>MSDREFVTVDPVTIIIKECINLSTAMRKYSKFTSQSGVAALLGGGSEIFSNQDDYLAHTFNNLNTNKHNDPFLSGFIQLRLMLNKLKNLDNIDSLTILQPFLLIVSTSSISGYITSLALDSLQKFFTLNIINESSQNYIGAHRATVNALTHCRFEGSQQLSDDSVLLKVVFLLRSIVDSPYGDLLSNSIIYDVLQTILSLACNNRRSEVLRNAAQSTMIAVTVKIFSKLKTIEPVNVNQIYINDESYTNDVLKADTIGTNVESKEEGSQEDPIGMKVNNEEAISEDDGIEEEHIHSEKSTNGAEQLDIVQKTTRSNSRIQAYADDNYGLPVVRQYLNLLLSLIAPENELKHSYSTRIFGLELIQTALEISGDRLQLYPRLFTLISDPIFKSILFIIQNTTKLSLLQATLQLFTTLVVILGNNLQLQIELTLTRIFSILLDDGTANNSSSENKNKPSIIKELLIEQISILWTRSPSFFTSTFINFDCNLDRADVSINFLKALTKLALPESALTTTESVPPICLEGLVSLVDDMFDHMKDIDREEFGRQKNEMEILKKRDRKTEFIECTNAFNEKPKKGIPMLIEKGFIASDSDKDIAEFLFNNNNRMNKKTIGLLLCHPDKVSLLNEYIRLFDFSGLRVDEAIRILLTKFRLPGESQQIERIIEAFSSAYCENQDYDPSKISDNAEDDISTVQPDADSVFILSYSIIMLNTDLHNPQVKEHMSFEDYSGNLKGCCNHKDFPFWYLDRIYCSIRDKEIVMPEEHHGNEKWFEDAWNNLISSTTVITEIKKDTQSVMDKLTPLELLNFDRAIFKQVGPSIVSTLFNIYVVASDDHISTRMITSLDKCSYISAFFDFKDLFNDILNSIAKGTTLINSSHDDELSTLAFEYGPMPLVQIKFEDTNTEIPVSTDAVRFGRSFKGQLNTVVFFRIIRRNKDPKIFSKELWLNIVNIILTLYEDLILSPDIFPDLQKRLKLSNLPKPSPEISINKSKESKGLLSTFASYLKGDEEPTEEEIKSSKKAMECIKSSNIAASVFGNESNITADLIKTLLDSAKTEKNADNSRYFEAELLFIIELTIALFLFCKEEKELGKFILQKVFQLSHTKGLTKRTVRRMLTYKILLISLCADQTEYLSKLINDELLKKGDIFTQKFFATNQGKEFLKRLFSLTESEFYRGFLLGNENFWKFLRKVTAMKEQSESIFEYLNESIKTDSNILTNENFMWVLGLLDEISSMGAVGNHWEIEYKKLTESGHKIDKENPYKKSIELSLKSIQLTSHLLEDNNDLRKNEIFAIIQALAHQCINPCKQISEFAVVTLEQTLINKIEIPTNEMESVEELIEGGLLPLLNSSETQEDQKILISSILTIISNVYLHYLKLGKTSNETFLKILSIFNKFVEDSDIEKKLQQLILDKKSIEKGNGSSSHGSAHEQTPESNDVEIEATAPIDDNTDDDNKPKLSDVEKD[2x]

The budding yeast homologs of GBF1, named Gea1 and Gea2, localize to early and medial Golgi compartments where Arf1 activation orchestrates the formation of COPI vesicles destined for the ER and earlier Golgi compartments. Here we present cryoelectron microscopy (cryoEM) structures of full-length Gea2, the yeast paralog of the human Arf-GEF GBF1, that reveal the organization of these regulatory domains and explain how Gea2 binds to the Golgi membrane surface. Gea2 and its paralogs possess an N-terminal DCB-HUS regulatory domain and C-terminal HDS1, HDS2, and HDS3 regulatory domains. The HDS1, −2, and −3 domains form an extended helical repeat structure that is contiguous with the DCB-HUS domain, such that the HDS3 domains of each monomer lie at the distal ends of the homodimer.

Three-dimensional classification of the particles revealed three distinct conformations of Gea2 homodimers that differed only in the positioning of the GEF domain, with each monomer adopting either a “closed” or “open” position relative to the regulatory domains. Based on the relative numbers of particle images that sorted into each of these three classes (~30% “closed/closed,” ~30% “open/open,” and ~40% “closed/open”), the conformation adopted by each monomer within the dimer appears to be largely independent of that of its binding partner. We begin our description of the structure using the “closed/open” dimer, as it exhibits both the closed and open states of the GEF domain. Unexpectedly, the GEF domain of Gea2 adopts two conformational states. The GEF domain lies adjacent to the HUS domain and is connected to the HUS and HDS1 domains through ordered linker regions. The conserved GEF-HDS1 linker adopts distinct conformations when in the closed, open, and Arf1-bound states and therefore appears important for stabilizing each of these states. Given the apparent independence of each GEF domain in the dimer, it is also possible that only one GEF domain is able to adopt the open conformation at a time when Gea2 is bound to the membrane. This possibility would enable the Gea2 dimer to remain more closely associated with the membrane surface throughout the activation reaction.> MRGSHHHHHHGMASNEFPVVLVINCGSSSIKFSVLDVATCDVLMAGIADGMNTENAFLSINGDKPINLAHSNYEDALKAIAFELEKRDLTDSVALIGHRIAHGGELFTQSVIITDEIIDNIRRVSPLAPLHNYANLSGIDAARHLFPAVRQVAVFDTSFHQTLAPEAYLYGLPWEYFSSLGVRRYGFHGTSHRYVSRRAYELLDLDEKDSGLIVAHLGNGASICAVRNGQSVDTSMGMTPLEGLMMGTRSGDVDFGAMAWIAKETGQTLSDLERVVNKESGLLGISGLSSDLRVLEKAWHEGHERARLAIKTFVHRIARHIAGHAASLHRLDGIIFTGGIGENSVLIRQLVIEHLGVLGLT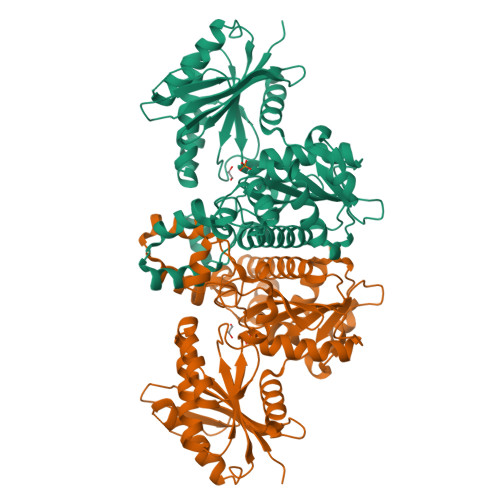LDVEMNKQPNSHGERIISANPSQVICAVIPTNEEKMIALDAIHLGNVKA> VVGGTDADEGEWPWQVSLHALGQGHICGASLISPNWLVSAAHCYI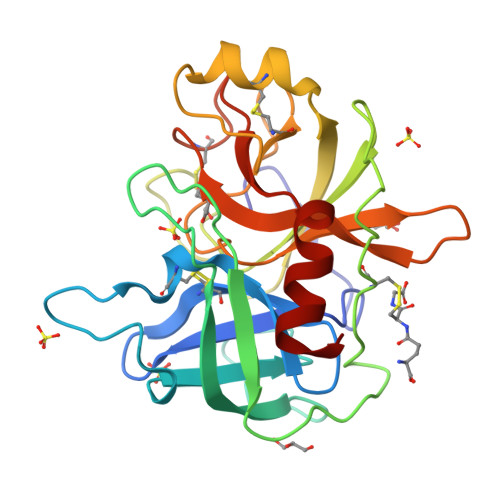DDRGFRYSDPTQWTAFLGLHDQSQRSAPGVQERRLKRIISHPFFNDFTFDYDIALLELEKPAEYSSMVRPICLPDASHVFPAGKAIWVTGWGHTQYGGTGALILQKGEIRVIQQTTCENLLPQQITPRMMCVGFLSGGVDSCQGDAGGPLSSVEADGRIFQAGVVSWGDGCAQRNKPGVYTRLPLFRDWIKENTGV>MINITSSASQEGTRLNLICTVWHKKEEAEGFVMFLCKDRSGDCSPETSLKQLRLKRDPGIDGVGEISSQLMFTISQVTPLHSGTYQCCARSQKSGIRLQGHFFSILFTETGN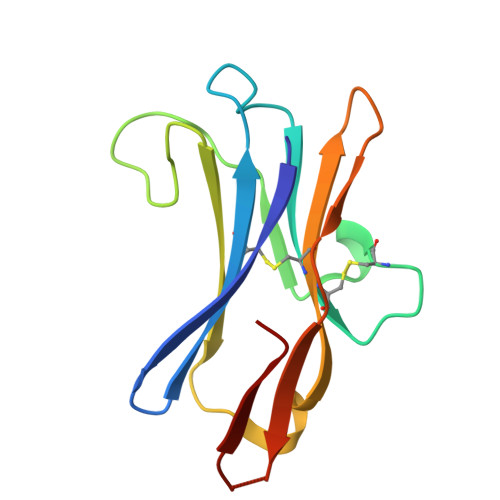YTVTGLK[2x]> MAASLGGMFTGQPPGPPPPPPGLPGQASLLQAAPGAPRPSNSTLVDELESSFEACFASLVSQDYVNGTDQEEIRTGVDQCIQKFLDIARQTECFFLQKRLQLSVQKPDQVIKEDVSELRSELQRKDALVQKHLT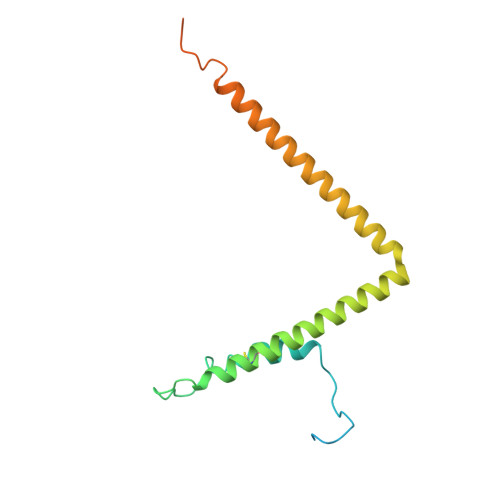KLRHWQQVLEDINVQHKKPADMPQGSLAFLEQASANIPAPLKQT[6-[[2,2-bis(fluoranyl)-1$l^{4},3-diaza-2$l^{4}-boratricyclo[7.3.0.0^{3,7}]dodeca-1(12),4,6,8,10-pentaen-8-yl]methyl]-2-azaspiro[3.3]heptan-2-yl]-[6-(3-cyclopropyl-1,2,4-triazol-1-yl)-2-azaspiro[3.3]heptan-2-yl]methanone 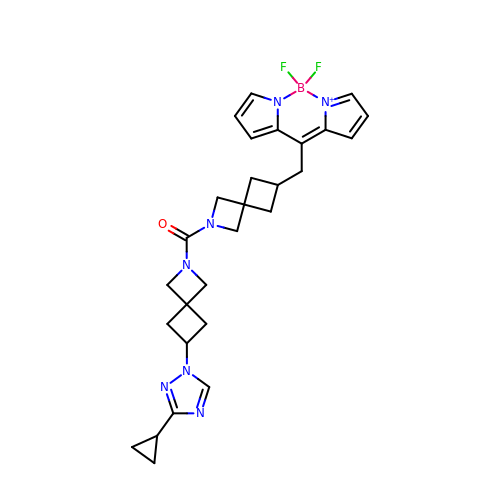| C28 H32 B F2 N7 O | PYTQGHQFGJMRKP-UHFFFAOYSA-N> GPHLICQSGDVLRARYEIVDTLGEGAFGKVVECIDHGMDG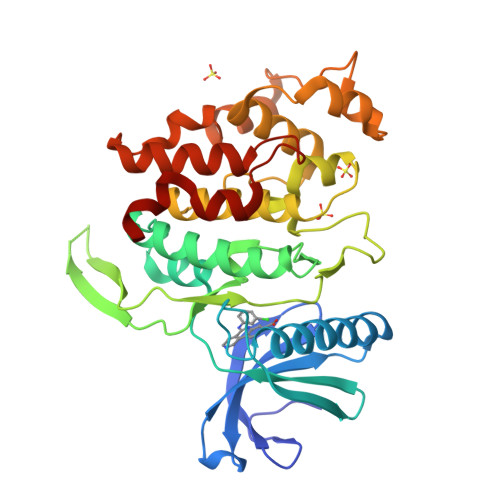MHVAVKIVKNVGRYREAARSEIQVLEHLNSTDPNSVFRCVQMLEWFDHHGHVCIVFELLGLSTYDFIKENSFLPFQIDHIRQMAYQICQSINFLHHNKLTHTDLKPENILFVKSDYVVKYNSKMKRDERTLKNTDIKVVDFGSATYDDEHHSTLVSTRHYRAPEVILALGWSQPCDVWSIGCILIEYYLGFTVFQTHDSKEHLAMMERILGPIPQHMIQKTRKRKYFHHNQLDWDEHSSAGRYVRRRCKPLKEFMLCHDEEHEKLFDLVRRMLEYDPTQRITLDEALQHPFFDLLKK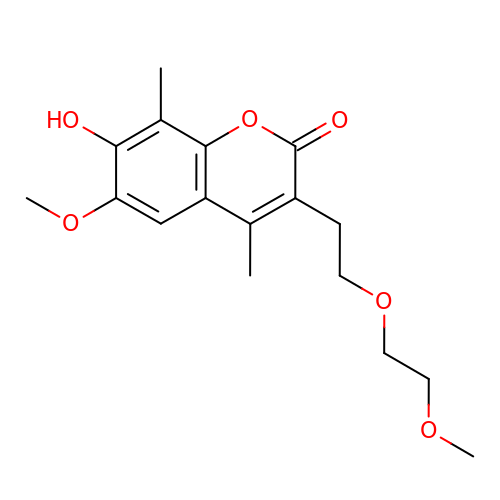7-hydroxy-6-methoxy-3-[2-(2-methoxyethoxy)ethyl]-4,8-dimethyl-2H-chromen-2-one | C17 H22 O6 | CREFVEORJKJSQY-UHFFFAOYSA-N6,7-dimethyl-2-sulfanylidene-1~{H}-pteridin-4-one 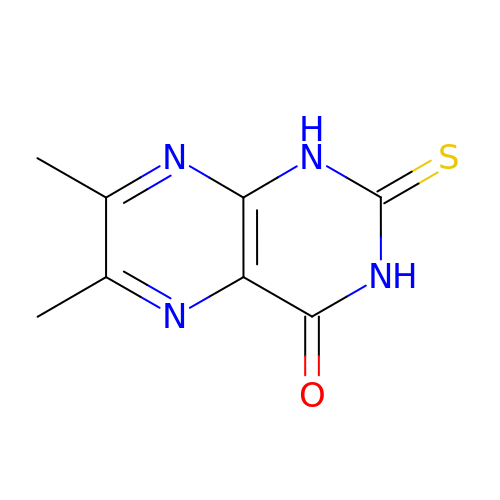| C8 H8 N4 O S | FMPVXDGAZOSEMT-UHFFFAOYSA-N> DSLSKSPENWMSKLDDGKHLTEINIPGSHDSGSFTLKDPVKSVWAKTQDKDYLTQMKSGVRFFDIRGRASADNMISVHHGMVYLHHELGKFLDDAKYYLSAYPNETIVMSMKKDYDSDSKVTKTFEEIFREYYYNNPQYQNLFYTGSNANPTLKETKGKIVLFNRMGGTYIKSGYGADTSGIQWADNATFETKINNGSLNLKVQDEYKDYYDKKVEAVKNLLA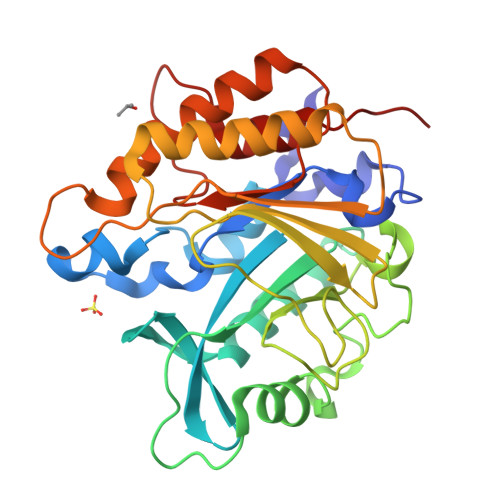KAKTDSNKDNVYVNFLSVASGGSAFNSTYNYASHINPEIAKTIKANGKARTGWLIVDYAGYTWPGYDDIVSEIIDSNKLEH> DPILLRPVDDLELTVRSANCLKAEAIHYIGDLV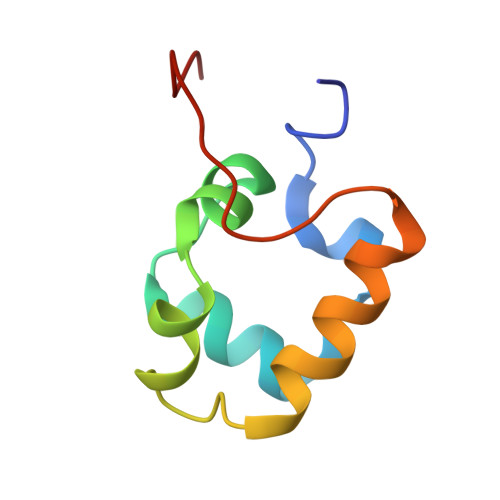QRTEVELLKTPNLGKKSLTEIKDVLASRGLSLGMRLENWPPA>[2x]ALIICYYGKNGAVIGGDRRQIFFRGSEENRKILEEKLYSGEIKSEEELYKLAEKLNIKIIIEDDREKVRKISDSVVCGEVRSLGIDAKRRRVYATKGKCAIVDILNDTV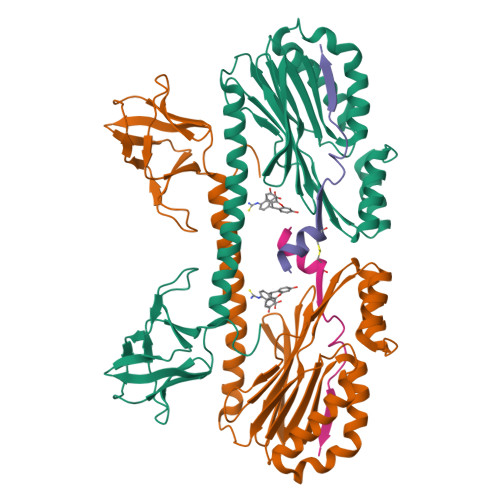TNQTIKEGFGIVVLGNRFLKKKAEEELKRTAKLFPMMPIQQIEDAIKEIFEKLKWHPTVSKEYDIYSVNKYEKNFEEVIKKDIESLFKYREQLRKQLIDFGKVMSIVNKIVKNGEIGVIKDGKLHLYDDYIAIDKIDPNPKVFKVVDVEGNFKDGDIVVIENGDMKIKGTNEKVTTKYIIIHKGSHHHHHH;>EDIGKITQAIKECLSKDPGAIDEDPFIIEL[2x]> XKKKKKK;> XEYEYEY

Here, we exploit IDRs to enable context-dependent heterotypic assemblies of intrinsically disordered peptides, where “context-dependent” refers to assembly behavior driven by interactions with other molecules. By attaching an aromatic segment to oppositely charged intrinsically disordered peptides, we achieve a nanofiber formation. Although the same-charged peptides cannot self-assemble, oppositely charged peptides form heterotypic nanofibers. pmcThis Communication reports the first cryo-EM structure of heterotypic assemblies formed by intrinsically disordered peptides and demonstrates their context-dependent assembly.

We selected KKKKKK as the positively charged intrinsically disordered peptide, a sequence found as a disordered region in proteins36−38 like KRas. We selected EYEYEY as the main negatively charged peptide for interacting with KKKKKK due to its presence in human proteins, such as MAP3K5, albeit without an experimentally verified ordered structure. Improved filament separation at pH 10 allowed for detailed imaging, showing a homogeneous, single type of cross-β filament with a diameter of ∼50 Å. Testing all possible indexed symmetries established that the nanofiber has C2 symmetry, with a helical rise of 4.68 Å and a twist of −4.22°, featuring parallel cross-β packing and six hydrophobic pyrene rings in the core. The nanofiber’s asymmetric subunit (ASU) contains three peptide copies: one Pyn-KKKKKK (1), one Pyn-EYEYEY (2), and a third with only an ordered pyrene ring. The remaining residues of the third peptide were flexible and disordered, revealing a disorder-to-order continuum and demonstrating unexpected conformational heterogeneity in heterotypic intrinsically disordered peptide nanofibers. Moreover, analysis of the atomic model revealed multiple hydrogen bonds between tyrosine and lysine, and we have seen side-chain densities from the cryo-EM map to support those side-chain conformations. K1 forms three intermolecular hydrogen bonds with Y2 and Y4 from the same peptide and Y2 from another peptide, and tyrosine also forms an intramolecular hydrogen bond between Y2 and Y4. The conformationally disordered Pyn-EYEYEY and Y6 from the ordered Pyn-EYEYEY should allow hydrogen bonding with additional Pyn-KKKKKK, which explains the postassembly bundle formation. To verify this, we also synthesized Pyn-EFEFEF to interact with Pyn-KKKKKK and found that postassembly addition of Pyn-KKKKKK was unable to form well-defined bundles.> MGSSHHHHHHSGDPFSECNDEIDNAKLIMKERRFTASYTFAKFSTGSMLLTKDIVGKSGVSIKRLPTELQRKFLFDDVYLDKEIEKVTIEARKSNPYPQISESSLLFKDALDYMEKTSSDYNLWKLSSILFDPVSYPYKTDNDQVKMALLKKERHCRLTSWIVSQIGPEIEEKIRNSSNEIEQIFLYLLLNDVVRASKLAIESKNGHLSVLISYLGSNDPRIRDLAELQLQKWSTGGCSIDKNISKIYKLLSGSPFEGLFSLKELESEFSWLCLLNLTLCYGQIDEYSLES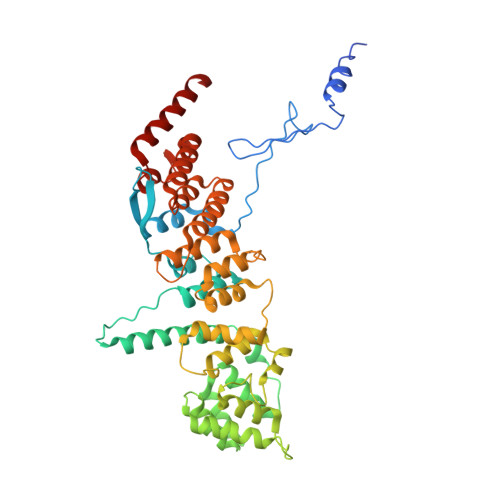LVQSHLDKFSLPYDDPIGVIFQLYAANENTEKLYKEVRQRTNALDVQFCWYLIQTLRFNGTRVFSKETSDEATFAFAAQLEFAQLHGHSLFVSCFLNDDKAAEDTIKRLVMREITLLRASTNDHILNRLKIPSQLIFNAQALKDRYEGNYL> MSNLSGTDKSVILLMTIGEDRAAEVFKHLSTREVQALSTAMANVRQISNKQLTDVLSEFEQEAEQFAALNINANEYLRSVLVKALGEERASSLLEDILETRDTTSGIETLNFMEPQSAADLIRDEHPQIIATILVHLKRSQ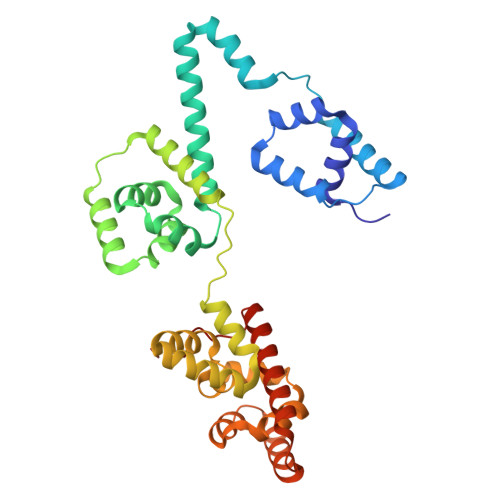AADILALFDERLRHDVMLRIATFGGVQLAELTEVLNGLLDGQNLKRSKMGGVRTAAEIINLMKTQQEEAVITAVREFDGELAQKIIDEMFLFENLVDVDDRSIQRLLQEVDSESLLIALKGAEPPLREKFLRNMSQRAADILRDDLANRGPVRLSQVENEQKAILLIVRRLAETGEMVIGSGEDTYV> G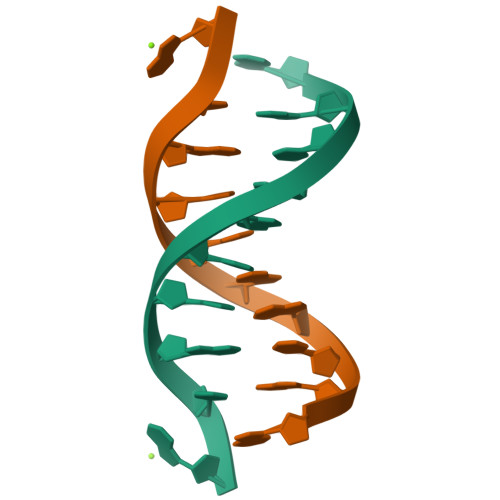GCAATTGCG> GM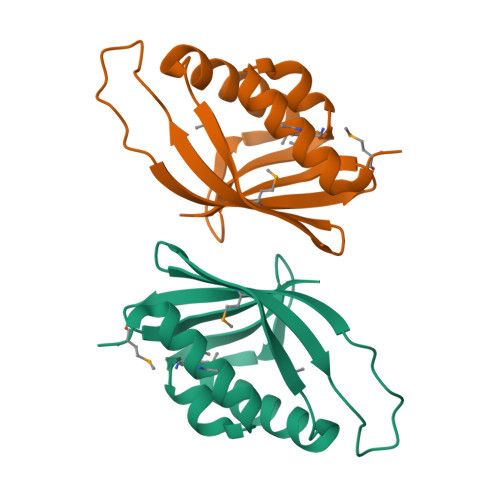SNLETAKAMIAAYNAQDVDTYVSYMTDDACEANYRGDVVREGKEGTRSGLAAAFARWPQNHAEIKDAQQVGTYVLMREHVTRGPATDGSPLVEPFDVVAVYSFEGDKCSRVEFIR>ETGMPQYSTFHSENRDWTFNHLTVHRRTGAVYVGAINRVYKLTGNLTIQVAHKTGPEEDNKACYPPLIVQPCSEVLTLTNNVNKLLIIDYSENRLLACGSLYQGVCKLLRLDDLFILVEPSHKKEHYLSSVNKTGTMYGVIVRSEGEDGKLFIGTAVDGKQDYFPTLSSRKLPRDPESSAMLDYELHSDFVSSLIKIPSDTLALVSHFDIFYIYGFASGGFVYFLTVQPETPDGMAINSAGDLFYTSRIVRLCKDDPKFHSYVSLPFGCTRAGVEYRLLQAAYLAKPGEALAQAFNISSDEDVLFAIFSKGQKQYHHPPDDSALCAFPIRAINLQIKERLQSCYHGEGNLELNWLLGKDVQCTKAPVPIDDNFCGLDINQPLGGSTPVEGLTLYTTSRDRLTSVASYVYNGYSVVFVGTKSGKLKKIRADGPPHGGVQYEMVSVFKDGSPILRDMAFSINQLYLYVMSERQVTRVPVESCEQYTTCGECLSSGDPHCGWCALHNMCSRRDKCQRAWEANRFAASISQCMSLEVHPNSISVSDHSRLLSLVVNDAPNLSEGIACAFGNLTEVEGQVSGSQVICISPGPKDVPVIPLDQDWFGLELQLRSKETGKIFVSTEFKFYNCSAHQLCLSCVNSAFRCHWCKYRNLCTHDPTTCSFQEGRINVSEDCPQLVPTEEILIPVGEVKPITLKARNLPQPQSGQRGYECVLSIQGAVHRVPALRFNSSSVQCQNSSYQYDGMDISNLAVDFAVVWNGNFIIDNPQDLKVHLYKCAAQRESCGLCLKADHKFECGWCSGERRCTLHQHCPSTSSPWLDWSSHNVKCSNPQITEILTVSGPPEGGTRVTIHGVNLGLDFSEIAHHVQVAGVPCTPIPGEYIIAEQIVCEMGHAVIGTTSGPVRLCIGECKPEFMTKSHQQYTFVNPSVLSLSPIRGPESGGTMVTITGHYLGAGSSVAVYLGNQTCEFYGRSMNEIVCVSPPSSNGLGPVPVSVSVDRARVDSSLQFEYIDDPRVQRIEPEWSITSGHTPLTITGFNLDVIQEPRVRVKFNGKESVNVCTVVNTTTLTCLAPSLTSDYRPGLDTVERPDEFGFLFNNVQSLLIYNDTKFIYYPNPTFELLSPTGILDQKPGSPIILKGKNLCPPASGGAKLNYTVMIGETPCT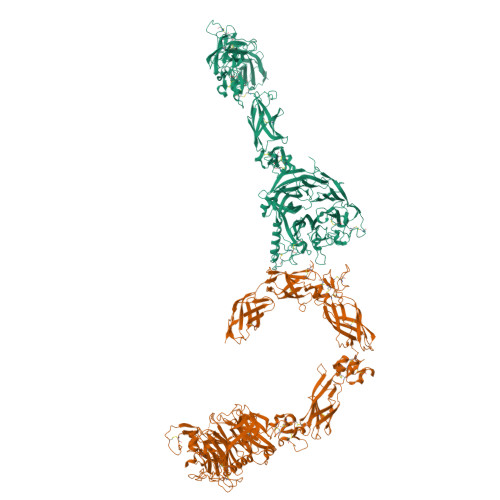VTVSETQLLCEPPNLTGQHKVMVHVGGMVFSPGSVSVISDGGSRTKHHHHHH[4x]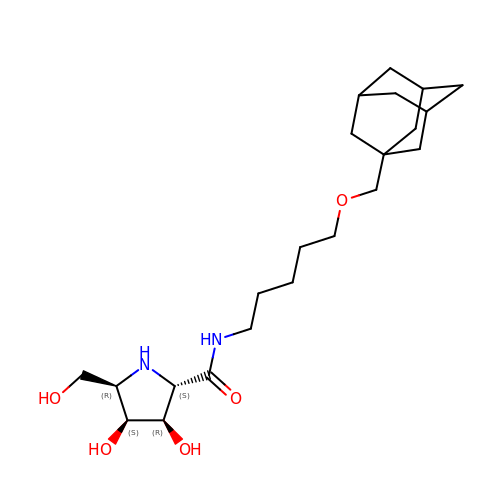(2~{S},3~{R},4~{S},5~{R})-~{N}-[5-(1-adamantylmethoxy)pentyl]-5-(hydroxymethyl)-3,4-bis(oxidanyl)pyrrolidine-2-carboxamide | C22 H38 N2 O5 | FWDXUUZGNWBLMB-HHSJJDFHSA-N> MASEAIKGAVVGIDLGTTNSCVAVMEGKQAKVLENAEGARTTPSVVAFTADGERLVGMPAKRQAVTNPNNTFYATKRLIGWRYDDPEVQKDIKNVPFKIVRASNGDAWVEAHGKLYSPSQIGAFVLMKMKETAENYLGHTAKNAVITVPAYFNDSQRQATKDAGQISGLNVLRVINEPTAAALAYGLDKSEDKVIAVYDLGGGTFDISILEIQKGVFEVKSTNGDTFLGGEDFDQALLRHIVKEFKRETGVDLTKDNMALQRVREAAEKAKCELSSSVQTDINLPYLTMDSSGPK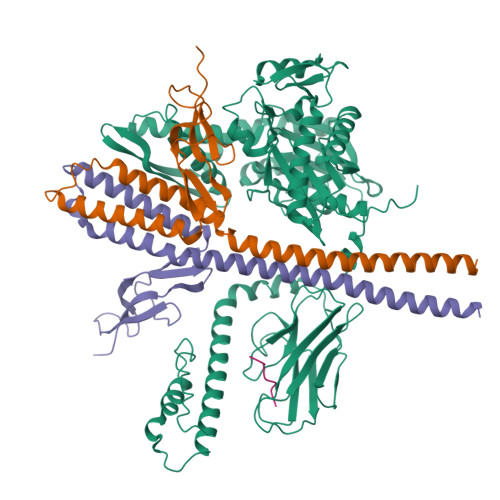HLNMKLTRAQFEGIVTDLIRRTIAPCQKAMQDAEVSKSDIGEVILVGGMTRMPKVQQTVQDLFGRAPSKAVNPDEAVAIGAAIQGGVLAGDVTDVLLLDVTPLSLGIETLGGVFTKLINRNTTIPTKKSQVFSTAADGQTQVEIKVCQGEREMAGDNKLLGQFTLIGIPPAPRGVPQIEVTFDIDANGIVHVSAKDKGTGREQQIVIQSSGGLSKDDIENMVKNAEKYAEEDRRKKERVEAVNMAEGIIHDTETKMEEFKDQLPADECNKLKEEISKMRELLARKDSETGENIRQAASS;>[2x]TLLEEKVKLEEQLKETVEKYKRALADTENLRQRSQKLVEEAKLYGIQAFCKDLLEVADVLEKATQCVPKEEIKDDNPHLKNLYEGLVMTEVQIQKVFTKHGLLKLNPVGAKFDPYEHEALFHTPVEGKEPGTVALVSKVGYKLHGRTLRPALVGVVKEASA;> VLLLDVT>[2x]MPPYTVVYFPVRGRC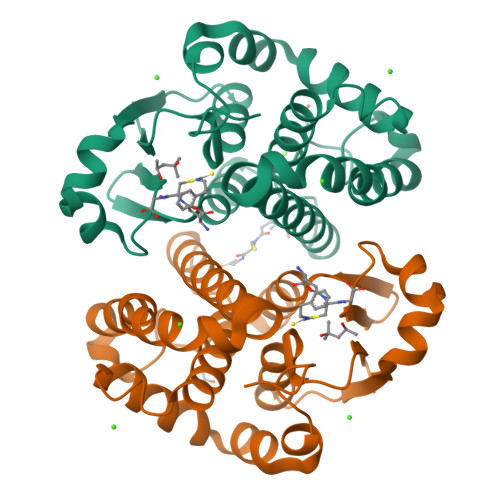AALRMLLADQGQSWKEEVVTVETWQEGSLKASCLYGQLPKFQDGDLTLYQSNTILRHLGRTLGLYGKDQQEAALVDMVNDGVEDLRCKYISLIYTNYEAGKDDYVKALPGQLKPFETLLSQNQGGKTFIVGDQISFADYNLLDLLLIHEVLAPGCLDAFPLLSAYVGRLSARPKLKAFLASPEYVNLPINGNGKQ> MKLDWEGRWNHVKKFLERSGPFTHPDFEPSTESLQFLLDTCKVLVIGAGGLGCELLKNLALSGFRQIHVIDMDTIDVSNLNRQFLFRPKDIGRPKAEVAAEFLNDRVPNCNVVPHFNKIQDFNDTFYRQFHIIVCGLDSIIARRWINGMLISLLNYEDGVLDPSSIVPLIDGGTEGFKGNARVILPGMTA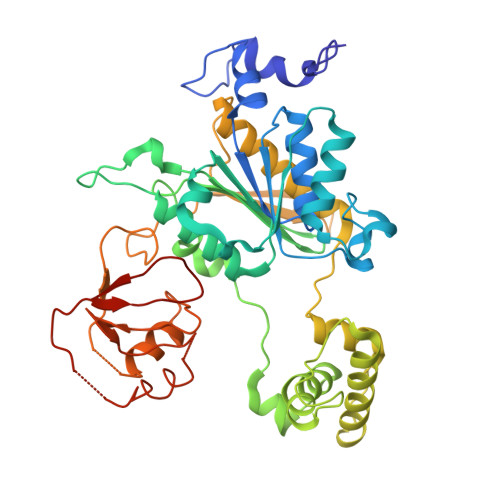CIECTLELYPPQVNFPMCTIASMPRLPEHCIEYVRMLQWPKEQPFGEGVPLDGDDPEHIQWIFQKSLERASQYNIRGVTYRLTQGVVKRIIPAVASTNAVIAAVCATEVFKIATSAYIPLNNYLVFNDVDGLYTYTFEAERKENCPACSQLPQNIQFSPSAKLQEVLDYLTNSASLQMKSPAITATLEGKNRTLYLQSVTSIEERTRPNLSKTLKELGLVDGQELAVADVTTPQTVLFKLHFTS> VGARRATYWAVLDTLVVGYALLPVLWIFSLSLKPTSTVKDGKLIPSTVTFDNYRGIFRGDLFSSALINSIGIGLITTVIAVVLGAMAAYAVARLEFPGKRLLIGAALLITMFPSISLVTPLFNIERAIGLFDTWPGLILPYITFALPLAIYTLSAFFREIPWDLEKAAKMDGATPGQAFRKVIVPLAAPGLVTAAILVFIFAWNDLLLALSLTATKAAITAPVAIANFTGSSQFEEPTGSIA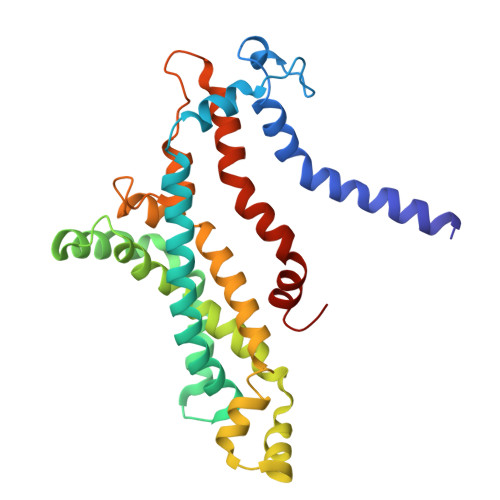AGAIVITIPIIVFVLIFQRRIVAGLTSGAVKG>MRTRSTISTPNGITWYYEQEGTGPDIVLVPDGLGECQMFDSSVSQIAAQGFRVTTFDMPGMSRSAKAPAETYTEVTAQKLASYVISILDALDIKHATVWGCSSGASTVVALLLGYPDRIRNAMCHELPTKLLDHLSNTAVLEDEEISNILANVMLNDVSGGSE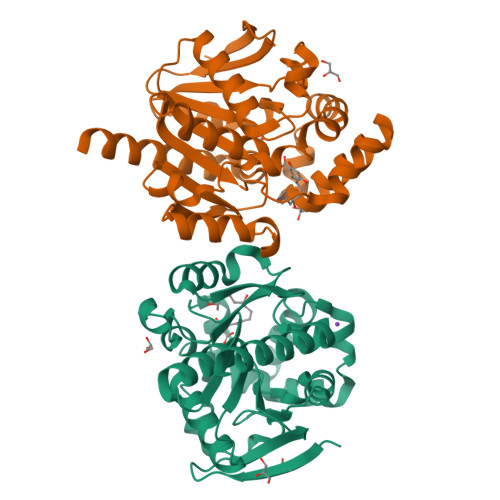AWQALGVEVHARLHKNYPVWARGYPRTIPPSAPVQDVEALRGKPLDWTVGAATPTESFFDNIVTATKAGVNIGLLPGMHFPYVSHPDVFAKYVVETTQKHLWNSSSVDKLAAALEHHHHHH[2x]P. gingivalis expresses two antigenically distinct but structurally homologous type-V fimbriae that are important both for attachment to other bacteria and for invasion of different host tissues. Instead, Mfa5 is the only fimbrial protein that has been found to be dependent on the type-IX secretion system for translocation across the outer membrane. Surprisingly, despite being unrelated in sequence, Mfa5 shows a striking similarity to the Gram-positive adhesins RrgA and GBS104, which both have a vWF domain and a number of IgG-like domains that appear to function as the stalk to project the VWF domain toward ligands, presumably those presented on host cells. Thus the vWF domain is a clear indication that the D1 domain of Mfa5 functions as an adhesin, but the ligand has yet not been determined.

However, no phase information could be obtained so a shorter construct, Mfa5138–435, encompassing only the predicted vWF domain was crystallized. One single rectangular crystal diffracting to 1.85 Å in space group P21 and with one molecule in the asymmetric unit was obtained. A highly redundant dataset was collected, and the structure was solved using sulfur SAD. The structure was refined to final Rwork and Rfree of 13 and 18%. The structure obtained from Mfa5138–435, that will be referred to as Mfa5D1, is folded into a vWF domain consisting of a typical Rossman fold comprising a six-stranded β-sheet surrounded by three helices on each side. This globular domain, which has a wrench-like form, has the dimensions 44 Å × 52 Å × 79 Å and includes the MIDAS motif, which is a central feature for interaction with various targets. In the Mfa5 MIDAS site, the five residues coordinating the metal ion are situated on the wrench head on top of the β-sheet. Mfa5 has a classical MIDAS motif36 in which the side chain oxygens of Ser152, Ser154, and Thr224 coordinate the metal directly and the side chains of Asp150 and Asp252 coordinate the metal via a water molecule. One of the loops in the ARM2 domain coordinates the second metal in the structure. Based on the coordination distances (average 2.4 Å), this metal has been modeled as a calcium ion.

> GAMAVTVPVDVVMVIDQSSSMGGQNIARLKSAIASGQRFVKKMLPKGMATEGVRIALVSYDHEPHRLSDFTKDTAFLCQKIRALTPIWGTHTQGGLKMARNIMATSTAVDKHIILMSDGLATEQYPVKNVTTADFIGETGNANDPIDLVIQGAINFPTNYVSNNPSTPLTPNYPTHSSKVGRRNLPESKFDYSNLSARITFDGVAGALVYEPRFPHPYYYYFPCNAAINEAQFAKNSGYTIHTIGYDLGDFALANNSLKLTATDENHFFTATPANLAAAFDNIAQTINIGIQRGEVTDFVA>[4x]MSAEQPTIIYTLTDEAPLLATYAFLPIVRAFAEPAGIKIEASDISVAARILAEFPDYLTEEQRVPDNLAELGRLTQLPDTNIIKLPNISASVPQLVAAIKELQDKGYAVPDYPADPKTDQEKAIKERYARCLGSAVNPVLRQGNSDRRAPKAVKEYARKHPHSMGEWSMASRTHVAHMRHGDFYAG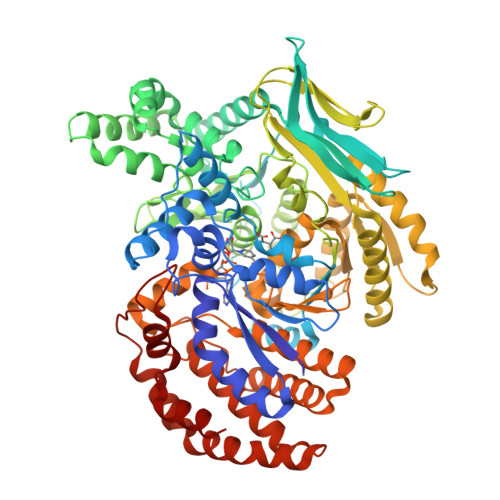EKSMTLDRARNVRMELLAKSGKTIVLKPEVPLDDGDVIDSMFMSKKALCDFYEEQMQDAFETGVMFSLHVKATMMKVSHPIVFGHAVRIFYKDAFAKHQELFDDLGVNVNNGLSDLYSKIESLPASQRDEIIEDLHRCHEHRPELAMVDSARGISNFHSPSDVIVDASMPAMIRAGGKMYGADGKLKDTKAVNPESTFSRIYQEIINFCKTNGQFDPTTMGTVPNVGLMAQQAEEYGSHDKTFEIPEDGVANIVDVATGEVLLTENVEAGDIWRMCIVKDAPIRDWVKLAVTRARISGMPVLFWLDPYRPHENELIKKVKTYLKDHDTEGLDIQIMSQVRSMRYTCERLVRGLDTIAATGNILRDYLTDLFPILELGTSAKMLSVVPLMAGGGMYETGAGGSAPKHVKQLVEENHLRWDSLGEFLALGAGFEDIGIKTGNERAKLLGKTLDAAIGKLLDNDKSPSRKTGELDNRGSQFYLAMYWAQELAAQTDDQQLAEHFASLADVLTKNEDVIVRELTEVQGEPVDIGGYYAPDSDMTTAVMRPSKTFNAALEAVQG> K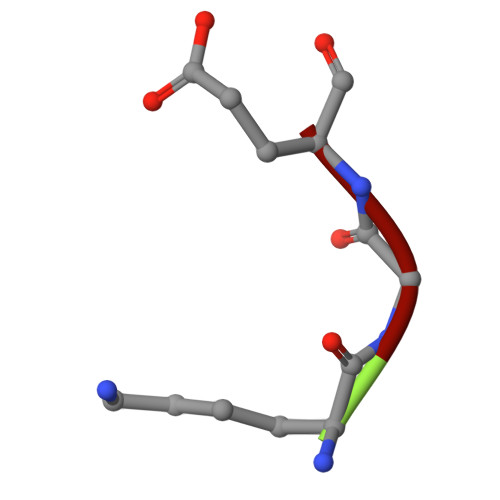GE> KETAA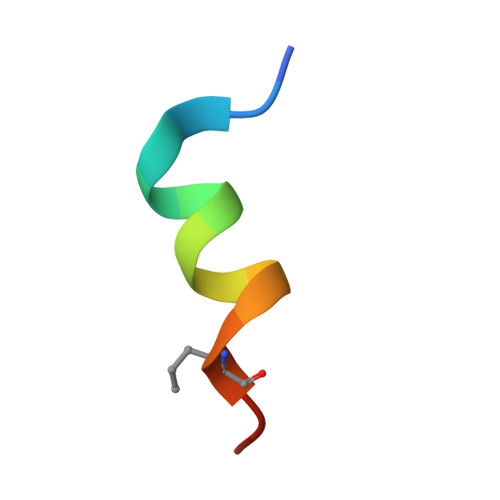AKFERQHLDSX>MGQGPELHLASQFVNEACRALVFGGCVEKSSVSRNPEVPFESSAYRISASARGKELRLILSPLPGAQPQQEPLALVFRFGMSGSFQLVPREELPRHAHLRFYTAPPGPRLALCFVDIRRFGRWDLGGKWQPGRGPCVLQEYQQFRENVLRNLADKAFDRPICEALLDQRFFNGIGNYLRAEILYRLKIPPFEKARSVLEALQQHRPSPELTLSQKIRTKLQNPDLLELCHSVPKEVVQLGGKGYGSESGEEDFAAFRAWLRCYGMPGMSSLQDRHGRTIWFQGDPGPLAPKGRKS[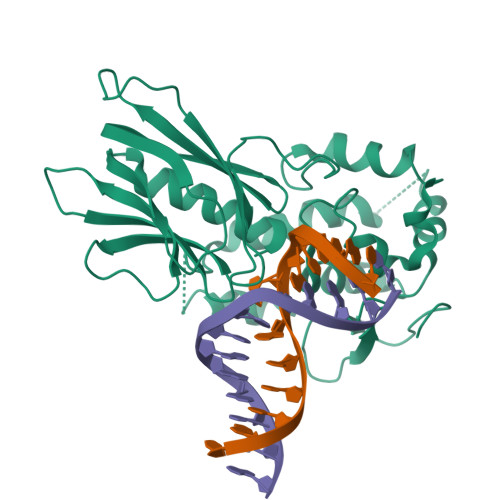2x]> GGATAA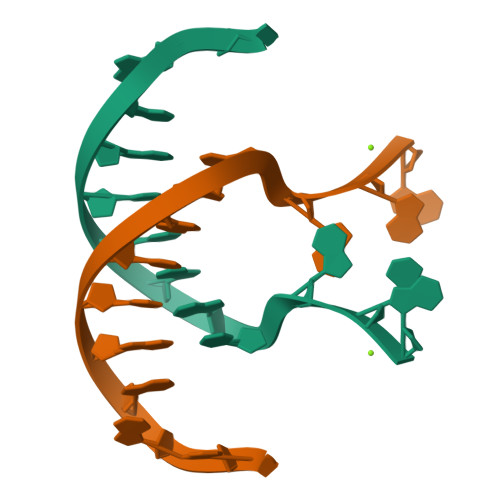TTAGGAG>[2x]AKVLISDSLDPCCRKILQDGGLQVVEKQNLSKEELIAELQDCEGLIVRSATKVTADVINAAEKLQVVGRAGTGVDNVDLEAATRKGILVMNTPNGNSLSAAELTCGMIMCLARQIPQATASMKDGKWERKKFMGTELNGKTLGILGL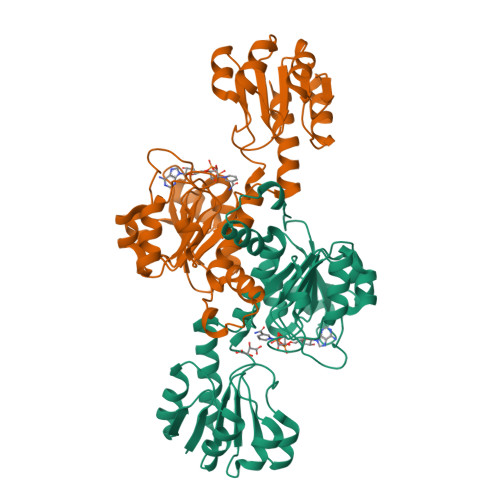GRIGREVATRMQSFGMKTIGYDPIISPEVSASFGVQQLPLEEIWPLCDFITVHTPLLPSTTGLLNDNTFAQCKKGVRVVNCARGGIVDEGALLRALQSGQCAGAALDVFTEEPPRDRALVDHENVISCPHLGASTKEAQSRCGEEIAVQFVDM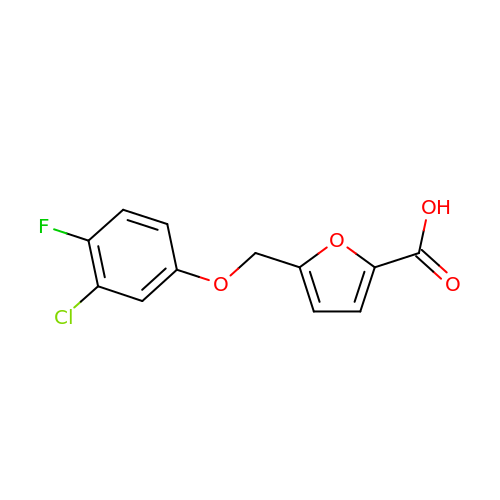5-[(3-chloranyl-4-fluoranyl-phenoxy)methyl]furan-2-carboxylic acid | C12 H8 Cl F O4 | UXWZMHGDRKKRHC-UHFFFAOYSA-N> GSYHADPSLVSFLTGLGCPNCIEYFTSQGLQSIYHLQNLTIEDLGAL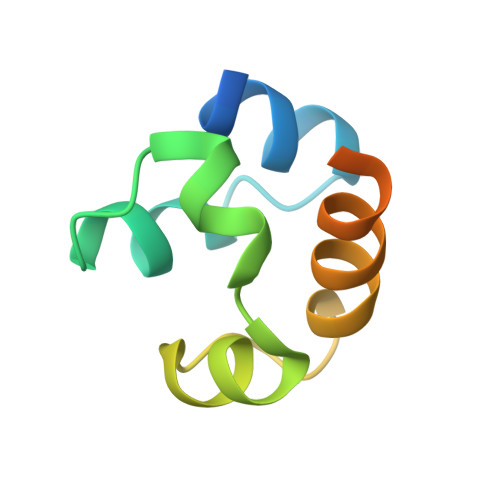KIPEQYRMTIWRGLQDLKQGHDYSTAQQLLRSS> DWISFSHMSSDTDHFPIKSWFRCEQKAASRSYRTLGDMSHPQGIYEVRAAITRLISLTRGVKCRPEQMIIGAGTQVLMQLLTELLPKEAVYAMEEPGYRRMYQLL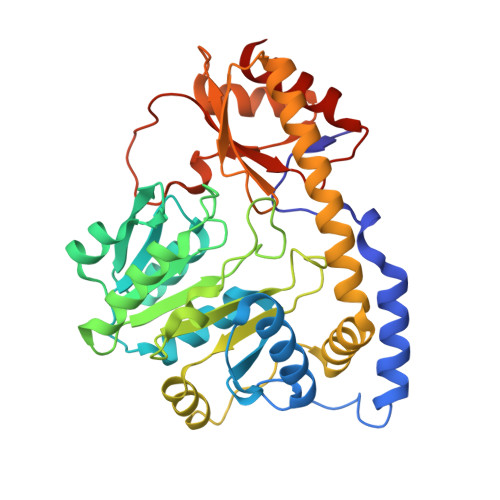KNAGKQVKTIMLDEKGMSIAEITRQQPDVLVTTPSHQFPSGTIMPVSRRIQLLNWAAEEPRRYIIEDDYDSEFTYDVDSIPALQSLDRFQNVIYMGTFSKSLLPGLRISYMVLPPELLRAYKQRGYDLQTCSSLTQLTLQEFIESGEYQKHIKKMKQHYKEKRERLITALEAEFSGEVTVKGANAGLHFVTEFDTRRTEQDILSHAAGLQLEIFGMSRFNLKENKRQTGRPALIIGFARLKEEDIQEGVQRLFKAVYG3,4-dihydroisoquinolin-1(2H)-one | C9 H9 N O | 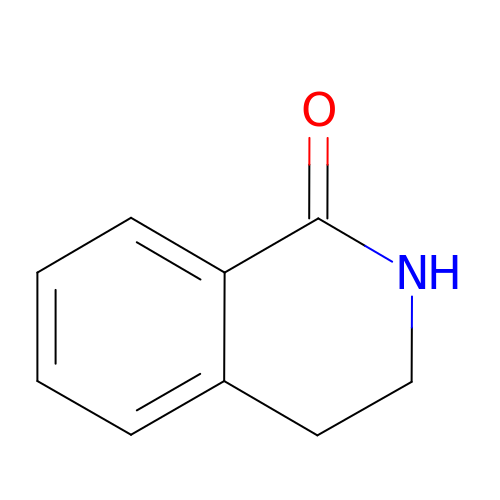YWPMKTWUFVOFPL-UHFFFAOYSA-N> HGYITFPIARQRRCNVQGGFWWPPDGSGIPDPMCRAAYQNVYNKVLQQGGTIDQAASAAQYMFQQDNEYAALAGPNYLDQNHIRNNVVPNYLCAAHATTWRIRPFGDKTGMDVSGSWTPTVIPLQDNTVSTVPIEFEFCPTAIHEPSFFEIYITVPSFNVYTDQVTWQQLINIFTGPIPLVQRRPDSQCNANNLVYRTTVGIPVRQTQFVLYVRWQRNDPVGEGFYNCADVIFAHRLGINEEDKIRPPKMKCKGNDKDCYKHHHRHNRYENDYENNYENYENYENNYENNYENNYENNYEYEYEYDRNNREHYHKCKHHSCMQHNYYERQYNTKDFNYVEWNDDYSDYIENHTGINRDMCDSTTKC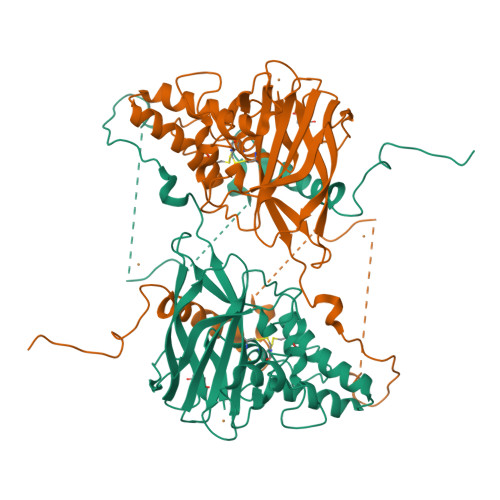CYK>MPGLFLTLEGLDGSGKTTQARRLAAFLEAQGRPVLLTREPGGGLPEVRSLLLTQELSPEAEYLLFSADRAEHVRKVILPGLAAGKVVISDRHLDSSLAYQGYGRGLPLPWLREVAREATRGLKPRLTFLLDLPPEAALRRVRRPDRLEGLGLEFFRRVREGYLALARAEPGRFVVLDATLPEEEIA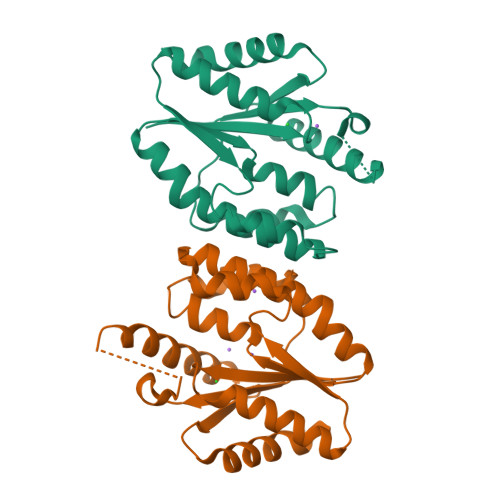RAIQAHLRPLLP[2x]> MEKSVSVILLAGGQGKRMKMSMPKQYIPLLGQPIALYSFFTFSRMPEVKEIVVVCDPFFRDIFEEYEESIDVDLSFAIPGKERQDSVYSGLQEIDVNSELVCIHDSARPLVNTEDVEKVLKDGSAVGAAVLGVPAKATIKEVNSDSLVVKTLDRKTLWEMQTPQVIKPELLKKGFELVKSEGLAVTDDVSIVEYLKHPVYVSQGSYTNIKVTTPDDLLLAERILSED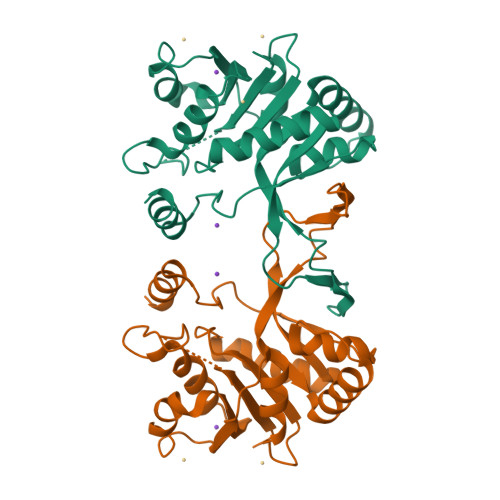S> ASPDDNFSPETLQFLRNNTGLDGEQWNNIMKLINKPEQDDLNWIKYYGYCEDIEDERGYTIGL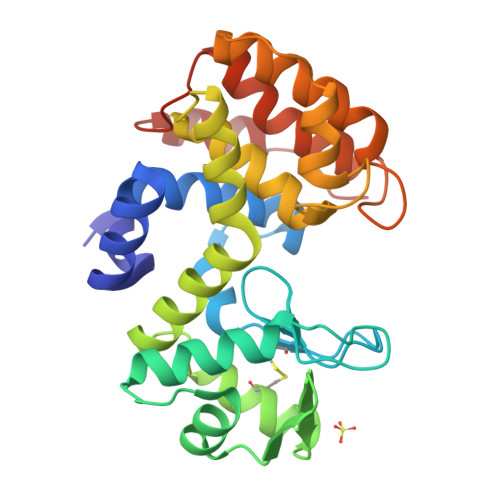FGATTGGSRDTHPDGPDLFKAYDAAKGASNPSADGALKRLGINGKMKGSILEIKDSEKVFCGKIKKLQNDAAWRKAMWETFYNVYIRYSVEQARQRGFTSAVTIGSFVDTALNQGATGGSDTLQGLLARSGSSSNEKTFMKNFHAKRTLVVDTNPYNKPPNGKNRVKQWDTLVDMGKMNLKNVDSEIAQVTDWEMK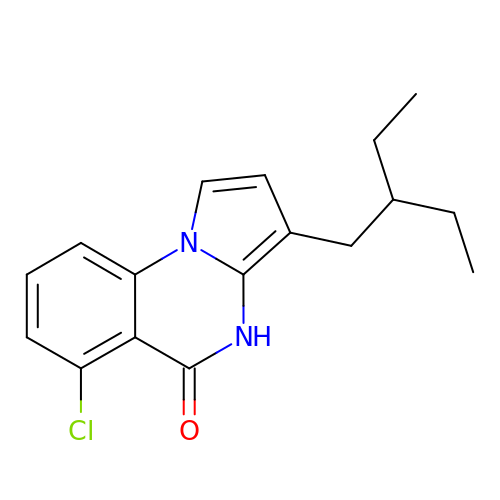6-chloranyl-3-(2-ethylbutyl)-4~{H}-pyrrolo[1,2-a]quinazolin-5-one | C17 H19 Cl N2 O | JCTQQDJVUAOWPC-UHFFFAOYSA-N>[4x]MLARKSIIPEEYVLARIAAENLRKPRIRDRLPKARFIAKSGACNLAHKNIREQGRFLQDIFTTLVDLKWRHTLVIFTMSFLCSWLLFAIMWWLVAFAHGDIYAYMEKGITEKSGLESAVCVTNVRSFTSAFLFSIEVQVTIGFGGRMMTEECPLAITVLILQNIVGLIINAVMLGCIFMKTAQAHRRAETLIFSRHAVIAVRNGKLCFMFRVGDLRKSMIISASVRIQVVKKTTTPEGEVVPIHQQDIPVDNPIESNNIFLVAPLIICHVIDKRSPLYDISATDLVNQDLEVIVILEGVVETTGITTQARTSYIA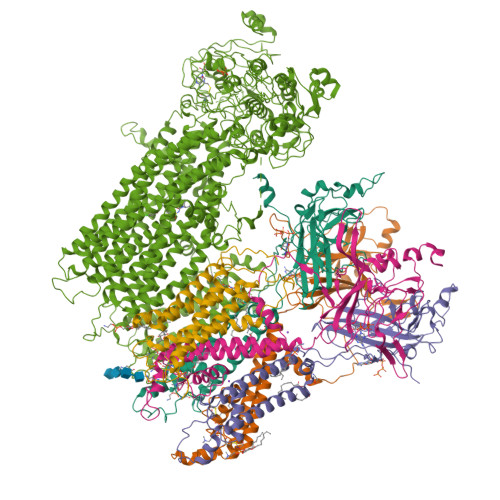EEIQWGHRFVSIVTEEEGVYSVDYSKFGNTVRVAAPRCSARELDEKPSILIQTLQKSELSHQNSLRKRNSMRRNNSMRRSNSIRRNNSSLMVPKVQFMTPEGNQCPSES;>MSLSFCGNNISSYNIYHGVLQNPCFVDALNLVPHVFLLFITFPILFIGWGSQSSKVQIHHNTWLHFPGHNLRWILTFALLFVHVCEIAEGIVSDSQRASRHLHLFMPAVMGFVATTTSIVYYHNIETSNFPKLLLALFLYWVMAFITKTIKLVKYWQLGWGMSDLRFCITGVMVILNGLLMAVEINVIRVRRYVFFMNPQKVKPPEDLQDLGVRFLQPFVNLLSKATYWWMNTLIISAHRKPIDLKAIGKLPIAMRAVTNYVCLKEAYEEQKKKAADHPNRTPSIWLAMYRAFGRPILLSSTFRYLADLLGFAGPLCISGIVQRVNEPKNNTTRFSETLSSKEFLENAHVLAVLLFLALILQRTFLQASYYVTIETGINLRGALLAMIYNKILRLSTSNLSMGEMTLGQINNLVAIETNQLMWFLFLCPNLWAMPVQIIMGVILLYNLLGSSALVGAAVIVLLAPIQYFIATKLAEAQKSTLDYSTERLKKTNEILKGIKLLKLYAWEHIFCKSVEETRMKELSSLKTFALYTSLSIFMNAAIPIAAVLATFVTHAYASGNNLKPAEAFASLSLFHILVTPLFLLSTVVRFAVKAIISVQKLNEFLLSDEIGEDSWRTGEGTLPFESCKKHTGVQSKPINRKQPGRYHLDNYEQARRLRPAETEDVAIKVTNGYFSWGSGLATLSNIDIRIPTGQLTMIVGQVGCGKSSLLLAILGEMQTLEGKVYWNNVNESEPSFEATRSRSRYSVAYAAQKPWLLNATVEENITFGSSFNRQRYKAVTDACSLQPDIDLLPFGDQTEIGERGINLSGGQRQRICVARALYQNTNIVFLDDPFSALDIHLSDHLMQEGILKFLQDDKRTVVLVTHKLQYLTHADWIIAMKDGSVLREGTLKDIQTKDVELYEHWKTLMNRQDQELEKDMEADQTTLERKTLRRAMYSREAKAQMEDEDEEEEEEEDEDDNMSTVMRLRTKMPWKTCWWYLTSGGFFLLFLMIFSKLLKHSVIVAIDYWLATWTSEYSINDPGKADQTFYVAGFSILCGAGIFLCLVTSLTVEWMGLTAAKNLHHNLLNKIILGPIRFFDTTPLGLILNRFSADTNIIDQHIPPTLESLTRSTLLCLSAIGMISYATPVFLIALAPLGVAFYFIQKYFRVASKDLQELDDSTQLPLLCHFSETAEGLTTIRAFRHETRFKQRMLELTDTNNIAYLFLSAANRWLEVRTDYLGACIVLTASIASISGSSNSGLVGLGLLYALTITNYLNWVVRNLADLEVQMGAVKKVNSFLTMESENYEGTMDPSQVPEHWPQEGEIKIHDLCVRYENNLKPVLKHVKAYIKPGQKVGICGRTGSGKSSLSLAFFRMVDIFDGKIVIDGIDISKLPLHTLRSRLSIILQDPILFSGSIRFNLDPECKCTDDRLWEALEIAQLKNMVKSLPGGLDATVTEGGENFSVGQRQLFCLARAFVRKSSILIMDEATASIDMATENILQKVVMTAFADRTVVTIAHRVHTILTADLVIVMKRGNILEYDTPESLLAQEDGVFASFVRADM[2x]>[2x]MQKDYQKLIVYLCDFLEKEVQKRGFKKVVYGLSGGLDSAVVGVLCQKVFKENAHALLMPSSVSMPENKTDALNLCEKFSIPYTE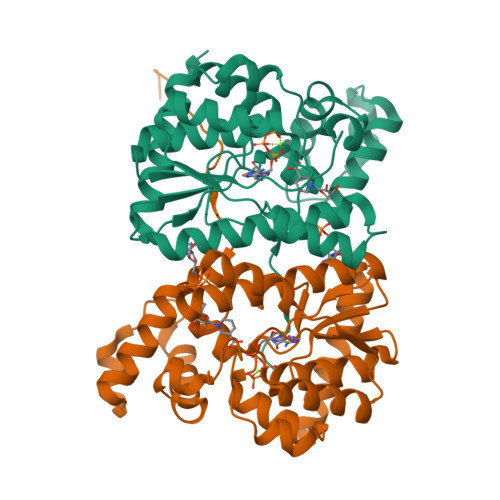YSIAPYDAIFSSHFKDASLTRKGNFCARLRMAFLYDYSLKSDSLVIGTSNKSERMLGYGTLFGDLACAINPIGELFKTEVYELARRLNIPKKILNKPPSADLFVGQSDEKDLGYPYSVIDPLLKDIEALFQTKPIDTETLAQLGYDEILVKNITSRIQKNAFKLELPAIAKRFNPELEHHHHHH Streptococcus mutans, a known etiological agent in the pathogenesis of dental caries, expresses three genetically distinct types of glucosyltransferases (Gtfs; also known as glucansucrases): GtfB (GTF-I), GtfC (GTF-SI) and GtfD (GTF-S). GtfC synthesizes both soluble and insoluble glucans (α-1,3 and α-1,6 glycosidic linkages), while GtfB and GtfD only synthesize insoluble glucans (mostly α-1,3 linkages) and soluble glucans (mostly α-1,6 linkages), respectively. All three enzymes belong to glycoside hydrolase family 70 (GH70), which cleaves the glycosidic bond between the glucose and fructose moieties in sucrose during catalysis. While fructose is released, the enzymatically produced glucose molecules are sequentially fused into a growing glucan chain and, depending on whether a 1,3- or 1,6-linkage is formed, the resultant product is either an insoluble or a soluble glucan, respectively.

Initially, GtfB-CD, like GtfD-CD, underwent proteolysis during crystallization setups at room temperature, which we only identified after the structures had been resolved since the gels after purification appeared to be satisfactory. Our attempts to stabilize GtfB-CD with protease inhibitors proved successful.

> AEQLNWLHFLMNFGNIYANDPDANFDSIRVDAVDNVDADLLQIAGDYLKAAKGIHKNDKAANDHLSILEAWSDNDTPYLHDDGDNMINMDNKLRLSLLFSLAKPLNQRSGMNPLITNSLVNRTDDNAETAAVPSYSFIRAHDSEVQDLIRDIIKAEINPNVVGYSFTMEEIKKAFEIYNKDLLATEKKYTHYNTALSYALLLTNKSSVPRVYYGDMFTDDGQYMAHKTINYEAIETLLKARIKYVSGGQAMRNQQVGNSEIITSVRYGKGALKATDTGDRTTRTSGVAVIEGNNPSLRLKASDRVVVNMGAAHKNQAYRPLLLTTDNGIKAYHSDQEAAGLVRYTNDRGELIFTAADIKGYANPQVSGYLGVWVPVGAAADQDVRVAASTAPSTDGKSVHQNAALDSRVMFEGFSNFQAFATKKEEYTNVVIAKNVDKFAEWGVTDFEMAPQYVSSTDGSFLDSVIQNGYAFTDRYDLGISKPNKYGTADDLVKAIKALHSKGIKVMADWVPDQMYAFPE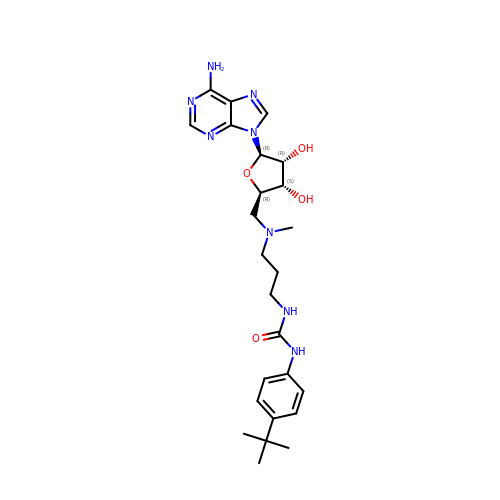5'-[(3-{[(4-tert-butylphenyl)carbamoyl]amino}propyl)(methyl)amino]-5'-deoxyadenosine | C25 H36 N8 O4 | DHTNDMXCZIAPMX-ZDXOVATRSA-N> GSLSWKRCAGCGGKIADRFLLYAMDSYWHSRCLKCSSCQAQLGDIGTSSYTKSGMILCRNDYIRLFGNSGACSACGQSIPASELVMRAQGNVYHLKCFTCSTCRNRLVPGDRFHYINGSLFCEHDRPTALINGHLNSGGSGGSGGSGGDVMVVGEPTLMGGEFGDEDERLITRLENTQFDAANGIDDE

In this paper, the advantages are explored of collecting X-ray anomalous data to identify chemical elements, such as metal ions, which are key to understanding certain structures and functions of proteins. By comparing anomalous peak heights or anomalous difference Fourier maps, specific elements can be identified and placed in the crystal structure. In this paper we used this method on three test crystals, LMO4, thermolysin and lysosyme, to identify zinc, calcium and chloride ions, respectively.

The anomalous peaks overlay with the previously modelled zinc ions. In the data set collected below the absorption edge, the theoretical zinc f′′ decreases to the level of sulfur (f′′ = 0.4 and 0.5 e− for sulfur and zinc, respectively), and both anomalous scatterers are visible in the anomalous difference Fourier maps. For each zinc-binding site, the anomalous peak heights decrease threefold between the data sets collected above and below the Zn K edge, confirming the presence of zinc. To illustrate the procedure, f′′ was refined with phenix.refine for the three collected LMO4 data sets. These data sets were initially collected to perform a three-wavelength multiple anomalous dispersion (MAD) experiment at peak (λ = 1.2853 Å), inflection (λ = 1.2874 Å) and remote (λ = 1.3051 Å) wavelengths. As the data sets were collected near the Zn K edge, significant variations in f′′ were observed over a short wavelength range. Nevertheless, the f′′ refinement successfully identified these variations, yielding values closely matching the measured values and confirming the validity of this approach.>GPLGSGAVQNTIERFTFPHKYKKRRPQDGKGKKDEGEESDTDEKCTICLSMLEDGEDVRRLPCMHL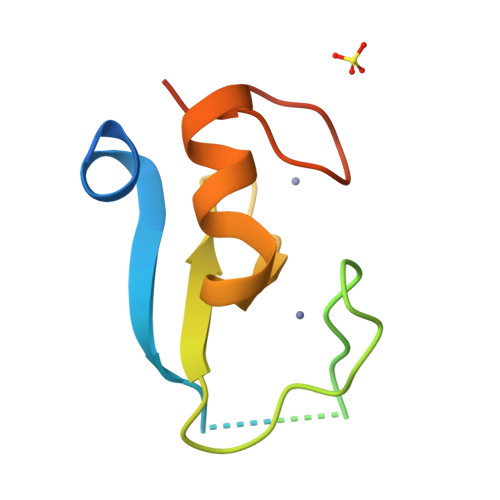FHQLCVDQWLAMSKKCPICRVDIETQLGADS[2x]> ESQPDPKPDELHKSSKFTGLMENMKVLYDDNHVSAINVKSIDQFLYFDLIYS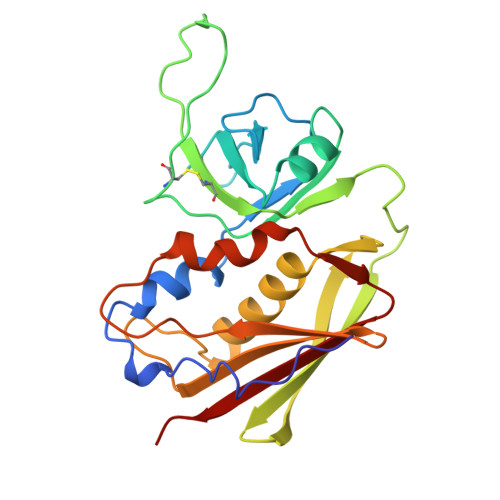IKDTKLGNYDNVRVEFKNKDLADKYKDKYVDVFGANYYYQCYFSKKTNDINSHQTDKRKTCMYGGVTEHNGNQLDKYRSITVRVFEDGKNLLSFDVQTNKKKVTAQELDYLTRHYLVKNKKLYEFNNSPYETGYIKFIENENSFWYDMMPAPGDKFDQSKYLMMYNDNKMVDSKDVKIEVYLTTKK> MLEAKFEEASLFKRIIDGFKDCVQLVNFQCKEDGIIAQAVDDSRVLLVSLEIGVEAFQEYRCDHPVTLGMDLTSLSKILRCGNNTDTLTLIADNTPDSIILLFEDTKKDRIAEYSLKLM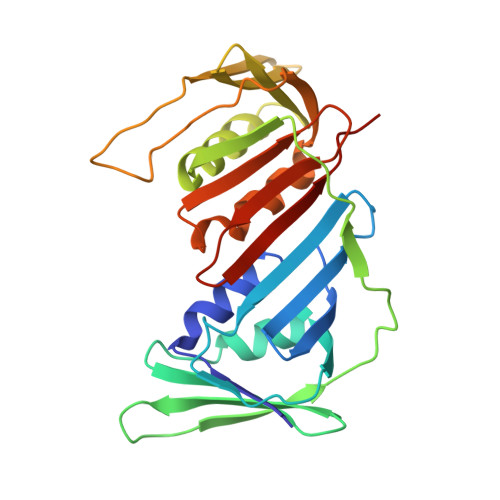DIDADFLKIEELQYDSTLSLPSSEFSKIVRDLSQLSDSINIMITKETIKFVADGDIGSGSVIIKPFVDMEHPETSIKLEMDQPVDLTFGAKYLLDIIKGSSLSDRVGIRLSSEAPALFQFDLKSGFLQFFLAPKFNDEE> MAFNDLLQQVGGVGRFQQIQVTLVVLPLLLMASHNTLQNFTAAIPTHHCRPPADANLSKNGGLEVWLPRDRQGQPESCLRFTSPQWGLPFLNGTEANGTGATEPCTDGWIYDNSTFPSTIVTEWDLVCSHRALRQLAQSLYMVGVLLGAMVFGYLADRLGRRKVLILNYLQTAVSGTCAAFAPNFPIYCAFRLLSGMALAGISLNCMTLNVEWMPIHTRACVGTLIGYVYSLGQFLLAGVAYAVPHWRHLQLLVSAPFFAFFIYSWFFIESARWHSSSGRLDLTLRALQRVARINGKREEGAKLSMEVLRASLQKELTMGKGQASAMELLRCPTLRHLFLCLSMLWFATSFAYYGLVMDLQGFGVSIYLIQVIFGAVDLPA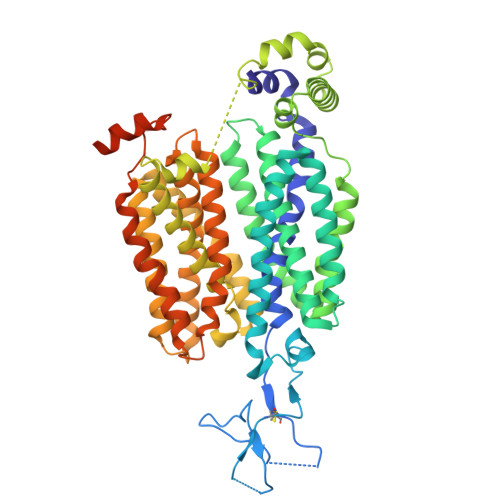KLVGFLVINSLGRRPAQMAALLLAGICILLNGVIPQDQSIVRTSLAVLGKGCLAASFNCIFLYTGELYPTMIRQTGMGMGSTMARVGSIVSPLVSMTAELYPSMPLFIYGAVPVAASAVTVLLPETLGQPLPDTVQDLESRWAPTQKEAGIYPRKGKQTRQQQEHQKYMVPLQASAQEKNGL4-methoxy-3-{[2-(piperidin-1-yl)-4-(trifluoromethyl)phenyl]sulfamoyl}benzoic 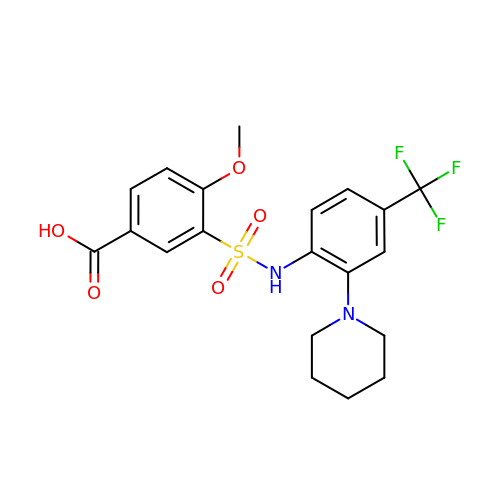acid | C20 H21 F3 N2 O5 S | BGLAMEXMBJAJBI-UHFFFAOYSA-N(6E,11E)-HEPTADECA-6,11-DIENE-9,9-DIYLBIS(PHOSPHONIC ACID) | C17 H34 O6 P2 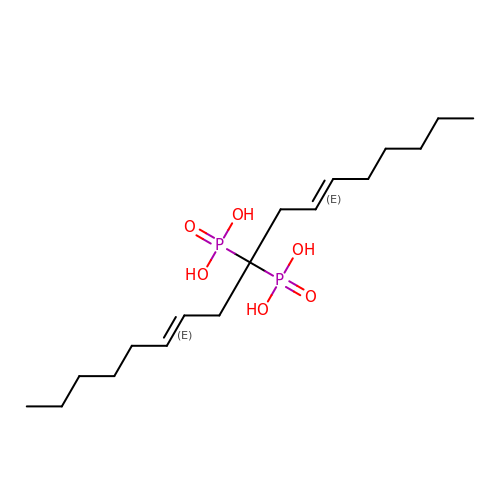| PFKBXXKNHWTTCS-PHEQNACWSA-N> SVVKVSLTHSASRMRVPEKRYGLAQTIESIKENVFTHFATPPEYMQLQLIDDRGITIEKNMANDKQLGY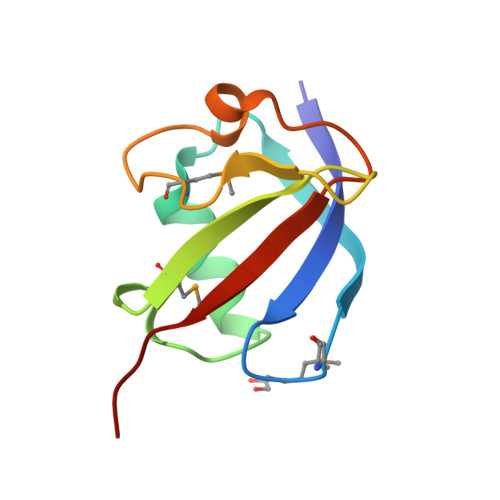YQCRDEFVIHVVDLQPS> SDLQRLKFIRHARQLGFSLESIRELLSIRIDPEHHTCQE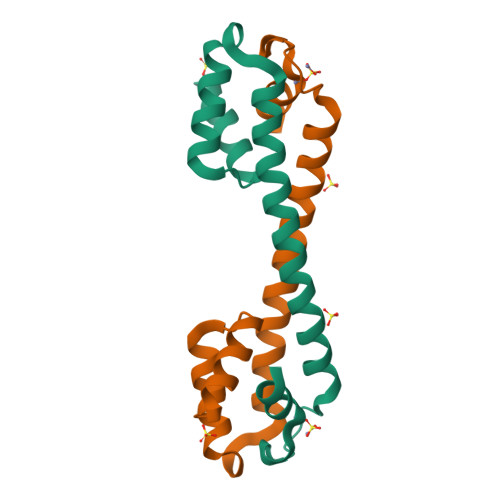SKGIVQERLQEVEARIAELQSMQRSLQRLNDACCGTAHSSVYCSILEALEQGASGVKSGC> MGLDSSHVGVRPSPATSQPTTST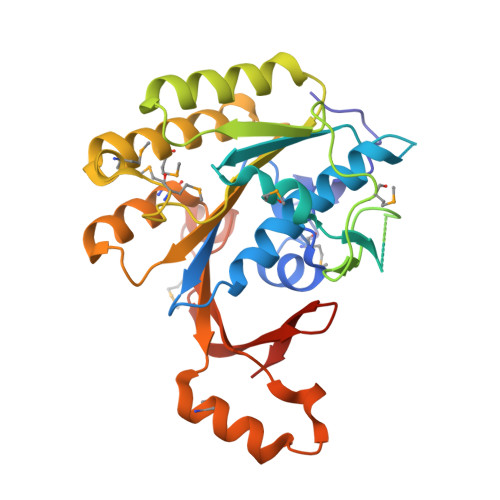GSADLDSILGHMGLPLGNSVLVEEQSTTEFHSILGKLFAAQGIVHNRISDSSADKTRNGDTHVIVLSLNQMFAKELPGIYKGSRKQMKKNLISEEESKVTVQNLNETQRSTPSRYKDLKIAWKYKLADEKRLGSPDRDDIQQNSEYKDYNHQFDITTRLMPAPIASELTFIAPTQPVSTILSQIEQTIKRNDKKLIRIVIPSLLHPAMYPPKMFESSEIIGLMHGVRSLVKKYYERVVLFASISIDIITPPLLVLLRNMFDSVINLEPFNQEMTEFLERVYKSQPGKIQHGLVHILKLPVFTDRGEMRVLKSEWAFKNGRKKFEIEQWGIPVDDAEGS> NIKQFNNMIQCTVPARSWWDFADYGCYCGSGSGSPVDDLDRCCQVHDNCYNAGGGVTGCAPKSKTYTYECSQGTLTCSGENSACAATVCDCDRLAAICFAGAPYNDNNY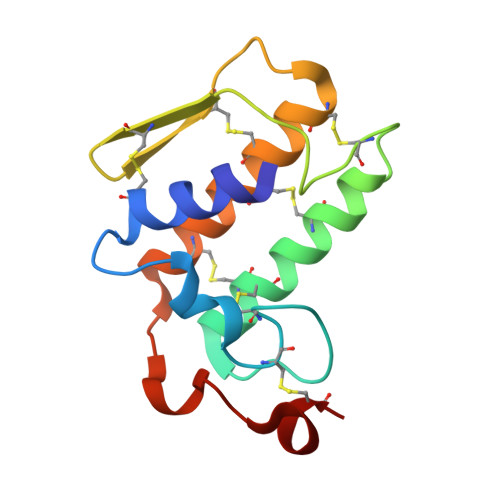NIDLKSRCQ> MQQQTLPKPFIWAEPHFMVPKEKQVTICCQGNYGAVEYQLHFEGSLFAVDRPKPPERINKVKFYIPDMNSRMAGQYSCIYRVGELWSEPSNLLDLVVTEMYDTPTLSVHPGPEVISGEK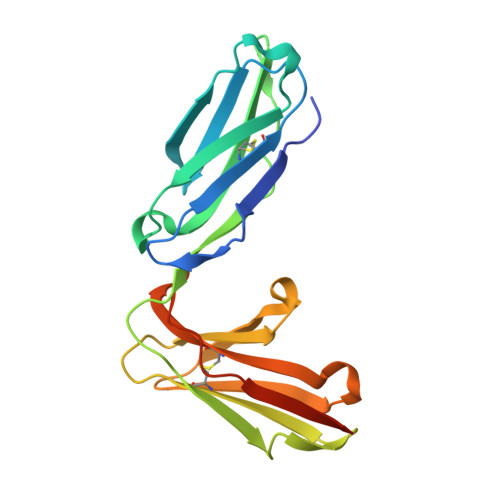VTFYCRLDTATSMFLLLKEGRSSHVQRGYGKVQAEFPLGPVTTAHRGTYRCFGSYNNHAWSFPSEPVKLLVTGDLEHHHHHH>ELGTGVDFPWAAVDNMMVRKGDTAVLRCYLEDGASKGAWLNR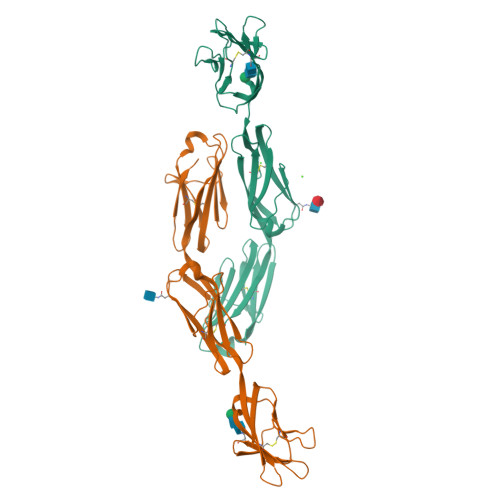SSIIFAGGDKWSVDPRVSISTLNKRDYSLQIQNVDVTDDGPYTCSVQTQHTPRTMQVHLTVQVPPKIYDISNDMTVNEGTNVTLTCLATGKPEPSISWRHISPSAKPFENGQYLDIYGITRDQAGEYECSAENDVSFPDVRKVKVVVNFAPTIQEIKSGTVTPGRSGLIRCEGAGVPPPAFEWYKGEKKLFNGQQGIIIQNFSTRSILTVTNVTQEHFGNYTCVAANKLGTTNASLPLNASTSHHHHHH[2x]> MSLKKGKFQHNQSKSLWNYTLSPGWREEEVKILKSALQLFGIGKWKKIMESGCLPGKSIGQIYMQTQRLLGQQSLGDFMGLQIDLEAVFNQNMKKQDVLRKNNCIINTGDNPTKEERKRRIEQNRKIYGLSAKQIAEIKLPKVKKHAPQYMTLEDIENEKFTNLEILTHLYNLKAEIVRRLAEQGETIAQPSIIKSLNNLNHNLEQN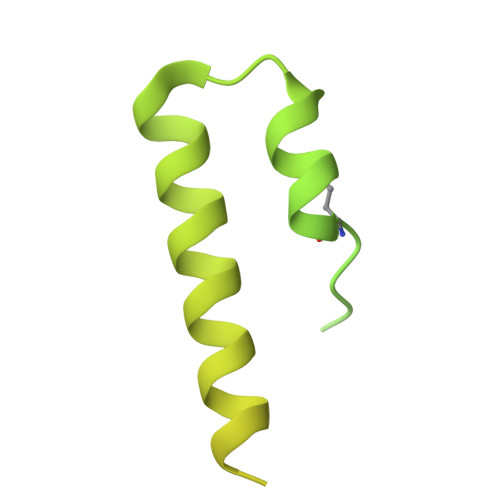QNSNSSTETKVTLEQSGKKKYKVLAIEETELQNGPIATNSQKKSINGKRKNNRKINSDSEGNEEDISLEDIDSQESEINSEEIVEDDEEDEQIEEPSKIKKR PrimPols are a class of primases that belong to the archaeo-eukaryotic primase (AEP) superfamily but have both primase and DNA polymerase activities. Replicative polymerase from NrS-1 phage (NrSPol) is a representative of the PrimPols. The domain organization of NrSPol is similar to that of ORF904, while the PrimPol domain of NrSPol lacks the typical zinc finger motif found in ORF904 and many other AEP family proteins, and the C-terminus of NrSPol has a unique helicase domain that forms a ring-shaped architecture and increases the polymerization activity of NrSPol. The processivity of NrSPol is dramatically enhanced when associated with NrS-1 phage-encoded helicase and ssDNA-binding protein, indicating that NrSPol is a replicative DNA polymerase capable of synthesizing the NrS-1 phage genome de novo.

In this study, to explore the structural basis of N300’s primase and primer extension functions, we determined the crystal structures of N300 in complex with ddCTP. The structure of N300 consists of two domains: a primase-like (Prim/Pol) domain located at the N-termini and a HBD at the C-termini. The two domains are connected by a linker region (178–195), of which electron density is missing due to flexibility. As is shown in Figure 1B, the primase-like domain adopts a saddle-shaped fold that resembles the previously reported PrimPol domain of ORF904 but with several significant differences. Frist, the primase-like domain of NrSPol utilizes a serine-rich loop with an SPS motif (S108, P109, and S110) instead of the very conserved zinc finger motif in the active site. Interestingly, the electron density of the S108 side chain extends to the γ-phosphate of ddCTP with a close O-O distance of 2.5 Å, suggesting a strong hydrogen bond. The side chain of S110 is also adjacent to the γ phosphate of ddCTP, with a O-O distance over 2.6 Å. This structure indicates that S108 and S110 coordinate ddCTP and are likely critical for N300’s primase and polymerase activities. Second, a chelated metal ion is found at the bottom of the N300 structure that is not present in any other PrimPol or primase structures. Given the high Ca2+ concentration in the crystal solution (100 mM), this metal ion is assigned as Ca2+, which is coordinated by the main chain carbonyl oxygens of T69, D72, F74, and E142.

> MIMEIPAIKALSRYAQWVIWKKERDTKIPYNPNNGKKASSTDPLAWGDIDEAQAGLVRYGANGLGFVLTKSDPFVFIDLDHVLDENKRVKCEWARQLLKEIKSYTEISPSGDGLHVVVSGKLPDYIKHKTKFDDGSALEVYESGRYMTITGEVFDGRDDIKELDLSILGEFAEHKIETKNAPVQIESATTLDDEAIIDLMKRKGQWPDAPADGDDWSSLDMSFANRLAFWCGKDIERMDRIFRQSPLMRQKWDRPTAGSTYGRITLKKACDFVDSVYDPALRNESDCPF> ATFEIVNRCS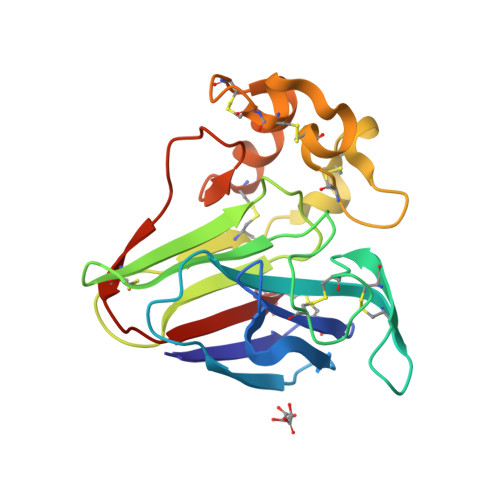YTVWAAASKGDAALDAGGRQLNSGESWTINVEPGTKGGKIWARTDCYFDDSGSGICKTGDCGGLLRCKRFGRPPTTLAEFSLNQYGKDYIDISNIKGFNVPMDFSPTTRGCRGVRCAADIVGQCPAKLKAPGGGCNDACTVFQTSEYCCTTGKCGPTEYSRFFKRLCPDAFSYVLDKPTTVTCPGSSNYRVTFCPTA>GSHMGRFADFFRIETEIQRLDNPAGILANGKKCDFTGACDPVVTAFLDLESPLSPWPGSVAASKWKTIFEATDQNSPTIGRSVIRDMCGGSASNVNLRVLVNDADSLSSQDEIGKFSCLFQLDARDVAMDSLSAQWGPSTECTAEAQQGKIRLFARRRAFEIPSTSCRAPSSL[2x]

Here, we show that a novel Mn-dependent peroxidase is an important factor in tardigrade anhydrobiosis. We crystallized the putative globular domain that lacked the N-terminus 62 amino acids of g12777 protein (g12777-Δ62) and solved the crystal structures as two forms containing Mn2+ or Zn2+ ions at 2.30 Å and 1.60 Å resolutions, respectively. The functional assays conducted here suggest that g12777 is a manganese-dependent peroxidase, independent of other components of the cell.

The Zn2+ g12777 protein structure was found to be bound to five Zn2+ ions originating from the crystallization buffer containing 300 mM zinc acetate, but not to Ca2+ from the protein buffer (2 mM calcium chloride). The Zn2+ crystal structure of putative catalytic domain (residues Gly63–Leu231) of the g12777 protein displayed a characteristic β-sandwich fold comprising seven β-strands and three 310 helices with three disulfide bridges (C91-C97, C146-C225, and C176-C200). As for the Zn2+-binding site located at the almost same region as that of Mn2+, the side-chain oxygen atoms of Asp92, Asp98, Asp161, and Asp163 coordinate with Zn2+ ion at distances of 1.9–2.0 Å. A considerable conformational difference was observed between Mn2+- and Zn2+-bound forms in terms of the metal-binding site, in which Asp92 and Asp98 were commonly involved in Mn2+ and Zn2+ binding. These aspartic acid residues were highly conserved within tardigrade orthologs, and the highly conserved CD-CD motif containing two Asp residues (D92 and D98) was used in the metal ion binding in both structures, suggesting the importance of these residues. The cysteine residues in this motif (C91 and C97) formed a disulfide bond in the crystal structure, suggesting that this disulfide bond may also contribute to this protein’s function. ITC experiment demonstrated that the estimated dissociation constants of the catalytic domain of the g12777 protein and Zn2+, Mn2+, and Ca2+ were 1.92 × 10–6 ± 6.00 × 10–8 M, 2.42 × 10–5 ± 1.75 × 10–6 M, or 1.39 × 10–4 ± 3.02 × 10–5 M, respectively, indicating that the binding affinity of Zn2+ was the highest among these divalent cations. Substitution of the Asp residues comprising Zn-1 (Asp92, Asp98, Asp161, and Asp163) to alanine (g12777-D2A) showed a decrease in cell survival, indicating that this binding site is required for antioxidative stress function. The recombinant β-sandwich domain of g12777 protein (g12777-Δ62) showed significant peroxidase activity when Mn2+ ions but not Zn2+ ions were present. We have also observed that the g12777 protein utilizes Mn2+ ions for peroxidase function, while it has a higher affinity for Zn2+ ions.B. bacteriovorus is an obligate bacterial predator of other Gram-negative bacteria, exploiting adaptations that allow consumption from inside the prey cell periplasm. The DgcB protein appends the C-terminal GGDEF enzymatic domain with an N-terminal forkhead-associated (FHA) domain, known to be used (in other proteins) for interactions with phosphopeptide ligands. DgcB comprised a ~30aa tail, 100aa FHA, 20aa linker and 160aa GGDEF domain. We provide the molecular basis for initiation of c-di-GMP production, demonstrating that the stimulus is a phosphopeptide tail present on the DgcB GGDEF synthase itself.

Distance constraints guided the assignment of FHA domains to their respective GGDEF partners, revealing a unique conformation for each chain. This arrangement is best described as a pseudosymmetrical GGDEF dimer, appended to two FHA domains that are asymmetrically orientated; the net effect is to place the FHA domains closer to GGDEF chain B. The dimer is stabilized by two molecules of c-di-GMP (classically intercalating via their planar bases), bound at the I-site of both monomers. The bound c-di-GMP arises from co-purification, as a result of (basally) active DgcB. The bound c-di-GMP dimer at the DgcB I-site is orientated in line with the two-fold axis of the GGDEF dimer, complexed by R218 and D221 of the conserved RxxD motif. The interactions of DgcB with the c-di-GMP ligand provide the major contact between the two GGDEF domains; direct protein:protein contacts are limited to just one weak interaction involving the partially ordered linker region. A putative N-terminal tail preceding the FHA domain (residues 1–31) is present on our construct but presumed disordered in this structure. Examination of the pocket reveals that the putative phosphate site is occupied by a bound ion in chain B, and that of chain A is partially occluded by residue D56. The vast majority of contacts to the GGDEF dimer are made by the chain A FHA domain; these comprises both polar (D70 and K48 to chain B) and non-polar (I40 and I126 to chain A, Y45 and Y68 to chain B) interactions. The conformation we observe likely represents a feedback-inhibited state wherein the GGDEF domain has been locked by the c-di-GMP product into a non-productive conformation; we posit that this represents a form present after entry of prey. Hence, most GGDEF proteins do not adopt this orientation as it would lead to steric clashes of the appended sensory domains, but in DgcB this conformation is enabled by having the chain B FHA domain offset.

>VPPAIVVLIGPPGYVGKQYPITASDIVIGRSVESQVYIDDKSLSRSHAKFAVNGSEVSVIDLGSTNKTIVNGQVIPPLASCLLKNNDQIKTGNVIFKFLEKGSIEAMTNAAMYDRAQKDALTGAHSKGALLDKGPEAMKRAEVLNEPFSLVTFDIDHFKKINDSYGHPGGDYVLKELCRIVITKLIRSNDFFARYGGEEFVLLLSGSPSKTAGEVGERIRQTIEAHDFTFEGKKIPVTISVGVATKLPNETEWTQVYDRADKALYQSKQGGRNRTTIVA[2x]> MIDYSGLRTIFGEKLPESHIFFATVAAHKYVPSYAFLRRELGLSSAHTNRKVWKKFVEAYGKAIPPAPPAPPLTLSKDLTASMSVEEGAALTLSVTATGGTGPYTYAWTKDGSPIPDASGATY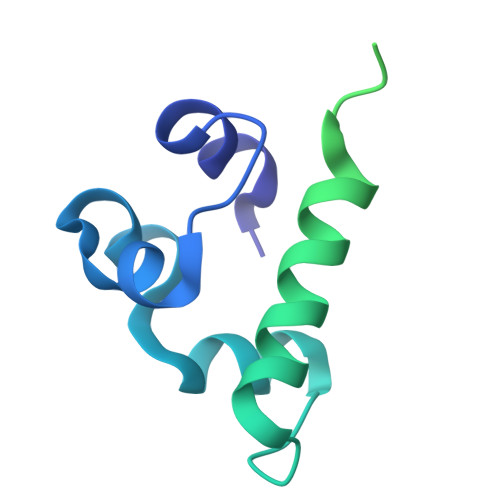TKPTAAAEDAGSYKVTVTDSKQVSKDSTTCAVTVNPTVPGG> MGSAFYKREM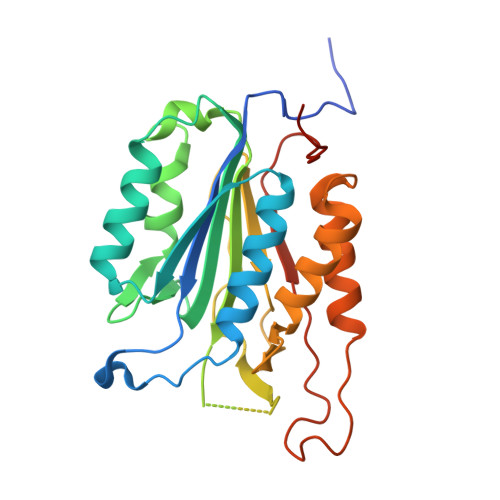FDPAEKYKMDHRRRGIALIFNHERFFWHLTLPERRGTCADRDNLTRRFSDLGFEVKCFNDLKAEELLLKIHEVSTVSHADADCFVCVFLSHGEGNHIYAYDAKIEIQTLTGLFKGDKCHSLVGKPKIFIIQAARGNQHDVPVIPLDVVDNQTEKLDTNITEVDAASVYTLPAGADFLMCYSVAEGYYSHRETVNGSWYIQDLCEMLGKYGSSLEFTELLTLVNRKVSQRRVDFCKDPSAIGKKQVPCFASMLTKKLHFFPKSNHHHHHH>MGSSHHHHHHSSGLVPRGSHMASATASRGASQAGAPQGRVPEARPNSMVVEHPEFLKAGKEPGLQIWRVEKFDLVPVPTNLYGDFFTGDAYVILKTVQLRNGNLQYDLHYWLGNECSQDESGAAAIFTVQLDDYLNGRAVQHREVQGFESATFLGYFKSGLKYKKGGVASGFKHVVPNEVVVQRLFQVKRRRVVRATEVPVSWESFNNGDCFILDLGNNIHQWCGSNSNRYERLKATQVSKGIRDNERSGRARVHVSEEGTEPEAMLQVLGPKPALPAGTEDTAKEDAANRKLAKLYKVSNGAGTMSVSLVADENPFAQGALKSEDCFILDHGKDGKIFVWKGKQANTEERKAALKTASDFITKMDYPKQTQVSVLPEGGETPLFKQFFKNWRDPDQTDGLGLSYLSSHIANVERVPFDAATLHTSTAMAAQHGMDDDGTGQKQIWRIEGSNKVPVDPATYGQFYGGDSYIILYNYRHGGRQGQIIYNWQGAQSTQDEVAASAILTAQLDEELGGTPVQSR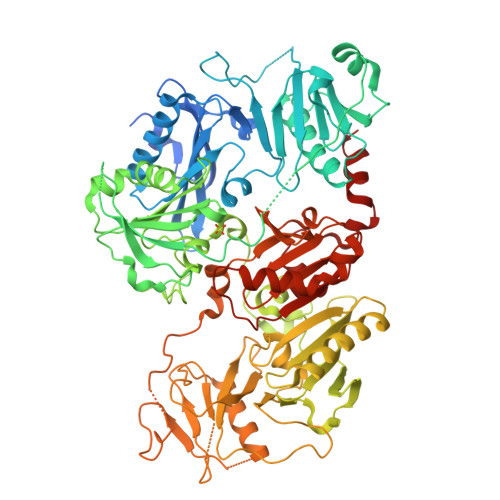VVQGKEPAHLMSLFGGKPMIIYKGGTSREGGQTAPASTRLFQVRANSAGATRAVEVLPKAGALNSNDAFVLKTPSAAYLWVGTGASEAEKTGAQELLRVLRAQPVQVAEGSEPDGFWEALGGKAAYRTSPRLKDKKMDAHPPRLFACSNKIGRFVIEEVPGELMQEDLATDDVMLLDTWDQVFVWVGKDSQEEEKTEALTSAKRYIETDPANRDRRTPITVVKQGFEPPSFVGWFLGWDDDYWSVDPLDRAMAELAA[2x]>MKNEKLAKGEMNLNALFIGDKAENGQLYKDLLIDLVDEHLGWRQNYMPQDMPVISSQERTSKSYEKTVNHMKDVLNEISSRMRTHSVPWHTAGRYWGHMNSETLMPSLLAYNFAMLWNGNNVAYESSPATSQMEEEVGHEFAHLMSYKNGWGHIVADGSLANLEGLWYARNIKSLPFAMKEVKPELVAGKSDWELLNMPTKEIMDLLESAEDEIDEIKAHSARSGKHLQAIGKWLVPQTKHYSWLKAADIIGIGLDQVIPVPVDHNYRMDINELEKIVRGLAEEQIPVLGVVGVVGSTEEGAVDSIDKIIALRDELMKDGIYYYVHVDAAYGGYGRAIFLDEDNNFIPYEDLQDVHEEYGVFKEKKEHISREVYDAYKAIELAESVTIDPHKMGYIPYSAGGIVIQDIRMRDVISYFATYVFEKGADIPALLGAYILEGSKAGATAASVWAAHHVLPLNVAGYGKLIGASIEGSHHFYNFLNDLTFKVGDKEIEVHTLTHPDFNMVDYVFKEKGNDDLVAMNKLNHDVYDYASYVKGNIYNNEFITSHTDFAIPDYGNSPLKFVNSLGFSDEEWNRAGKVTVLRAAVMTPYMNDKEEFDVY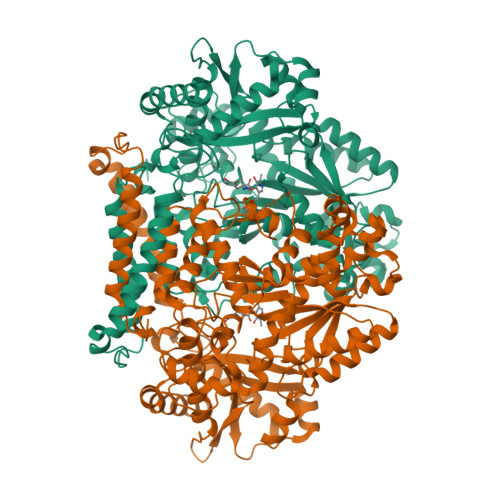APKIQAALQEKLEQIYDVK[3x]L. pneumophila encodes molecular mimics of host E3 ligases, including the effector protein RavN, thereby subverting the ubiquitylation pathway for its own benefit during infection. Using protein crystallography, we show that the fold of RavN has only residual resemblance to conventional eukaryotic E3s, yet its mode of interaction with E2 enzymes, host proteins that are important for the ubiquitin transfer reaction, has been preserved throughout evolution. When using RavN (Lpg1111; 212 amino acids, 24 kDa), a translocated substrate of the Dot/Icm Type IV secretion system (T4SS), as bait, a protein of approximately 35 kDa in size was highly enriched in the pulldown fraction but not in the control lanes. While control reactions lacking either GST-RavN or an E2 underwent no noticeable poly-ubiquitylation, efficient poly-ubiquitylation was detected upon incubation of GST-RavN with the E2 enzymes UbcH5a, UbcH5b, UbcH5c, and UbcH6, but none of the other E2s, indicating that RavN was indeed an E3 ubiquitin ligase that preferred a select set of host E2s.

Thus, we carried out limited trypsin-mediated proteolysis in combination with Matrix Assisted Laser Desorption/Ionization–Time of Flight (MALDI–TOF) mass spectrometry to identify stable fragments that may be more amenable to crystallization. This approach proved successful in producing a RavN fragment (residues 1–123; RavN1-123) that existed as a monomer in solution and that crystallized readily. The U-box domain resembled the zinc-finger-containing structure present in all RING domains, but lacked the Zn2+-coordinating sites which are substituted by a network of stabilizing hydrogen bonds and salt bridges. However, in the case of the RavN U-box domain, the position corresponding to αA is occupied by a segment of the loop L4 (residues 37–42; L4RavN) that connects the central β-hairpin with the equivalent loop L2E3 without altering its relative orientation. In fact, for all active RING-finger/U-box domains, the L1E3, L2E3 and αA elements create a conserved hydrophobic surface that serves as the docking site for E2 binding, as investigated for RavN below. The remaining three alpha helices (α1, α2 and α3) and the connecting loops (L5 and L6) are folded as a “cup” or “goblet” (colored slate in Fig 3A) that surrounds the base of the U-box domain. Superimposition of their structures with that of RavN revealed the presence of three residues in RavN (Ile8, Leu43 and Pro47) that create a surface area analogous to the E2 binding regions present in Ark2C and CHIP, suggesting that these residues could be important for E2 binding and, thus, E3 ligase activity of RavN. Notably, owing to crystal packing, helix α3 adopted multiple orientations among the three RavN1-123 molecules present within the asymmetric unit. The angles between different orientations of helix α3 ranged from 56° for α3A∠C to 134° for α3A∠B and 137° for α3B∠C.

>GAMGSMPTYFDPIMQEDTVLDENTIVYLVKIGDNKFSIKAISSGLEHLPSDPTTHAEKYWPIPAKSLIDHSSNKLLFEEDKLTNQPISKDQVIELFAVDPDKTEPKQFSDSVKRELTENWAREVLQDQ[3x]> GLGDELEEVIVEKTKQTVASISSGPKHTQKVPILTANETGATMPVLPSDSIETRTTYMHFNGSETDVECFLGRAACVHVTEIQNKDATGIDNHREAKLFNDWKINLSSLVQLRKKLELFTY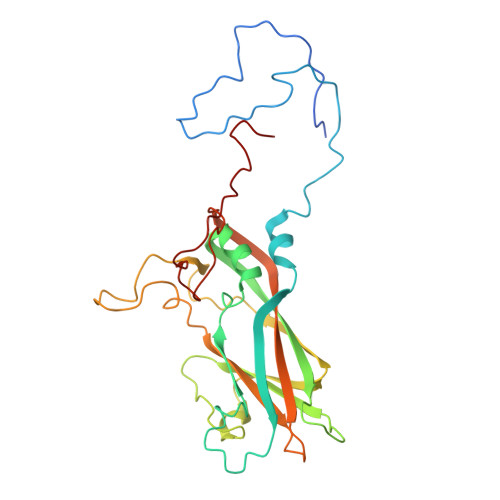VRFDSEYTILATASQPDSANYSSNLVVQAMYVPPGAPNPKEWDDYTWQSASNPSVFFKVGDTSRFSVPYVGLASAYNCFYDGYSHDDAETQYGITVLSHMGSMAFRIVNEHDEHKTLVKIRVYHRAKHVEAWIPRAPRALPYTSIGRTNYPKNTEPVIKKRKGDIKSY>MIDLIVSQGRVADRAAWMIEGAARTARALEERYGLKGHYVGEPAPHADDDWSVALPQARETLVAVREAATESIKGDNLTVLVNNTCSVSLATLPVVAREHPDAVVLYIDGHGDFNTPETTDTGYLGGMVLSGACGLWDSGHGAGLRPEQAVLVGSRDIDEGERELIRKAGVRV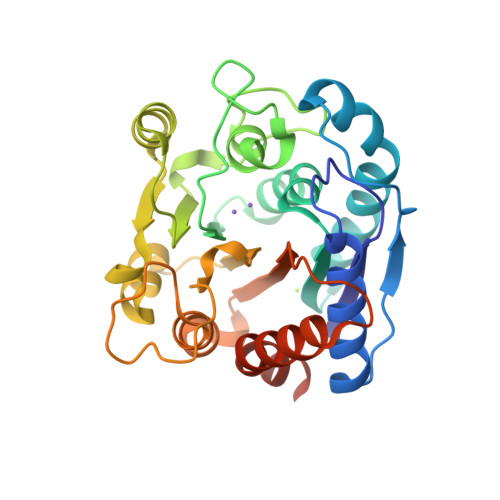IPPGEATAQAVLDAVKDAPVWIHIDWDVLEPGSIPADYTVPDGMLPAQIRAVFEAIPAERLIGVELAELNAPADSERAEQAVAVILDMVAPAFDAAAARPLEHHHHHH[2x]> GAEFMAVAGAVSGEPLVHWCTQQLRKTFGLDVSEEIIQYVLSIESAEEIREYVTDLLQGNEGKKGQFIEELITKWQKNDQELISDPLQQCFKKDEILDGQKSGDHLKRGRKKGRNRQEVPAFTEPDTTAEVKTPFDLAKAQENSNSVKKKTKFVNLYTREGQDRLAVLLPGRHPCDCLGQKHKLINNCLICGRIVCEQEGSGPCLFCGTLVCTHEEQDILQRDSNKSQKLLKKLMSGVENSGKVDISTKDLLPHQELRIKSGLEKAIKHKDKLLEFDRTSIRRTQVIDDESDYFASDSNQWLSKLERETLQKREEELRELRHASRLSKKVTIDFAGRKILEEENSLAEYHSRLDETIQAIANGTLNQPLTKLDRSSEEPLGVLVNPNMYQSPPQWVDHTGAASQKKAFRSSGFGL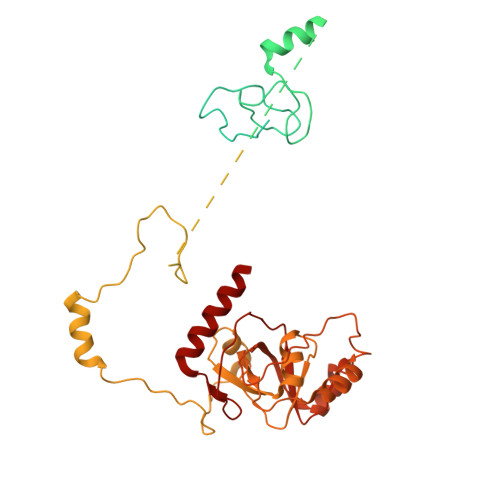EFNSFQHQLRIQDQEFQEGFDGGWCLSVHQPWASLLVRGIKRVEGRSWYTPHRGRLWIAATAKKPSPQEVSELQATYRLLRGKDVEFPNDYPSGCLLGCVDLIDCLSQKQFKEQFPDISQESDSPFVFICKNPQEMVVKFPIKGNPKIWKLDSKIHQGAKKGLMKQNKAV>GSARLKGITLRIGVIESVPFTIVANVIDTSGRNTTKLTGYVLDLIEYLRDKMGFVADVQLAPPNTSYTGLVLALANGDYDIAIGDITVTSARREIVAFSNSISDNSMRILMRKGTLIDGMDDLKNGKIPYNRIGIRIGTAGEDYYLREISGGSRNFYPLKSRQEMYDSLLAGIIDVSFMDIGTAEYVTNNIYCNLTLVGEDF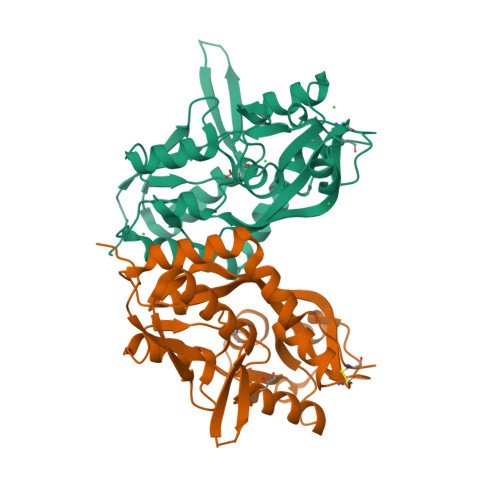DKSTFGIVTPKEWLYAKDLDVNILSLRETGILDNLKKKWFQTKACP[2x]>GPLGSKKLKCTVEGCDR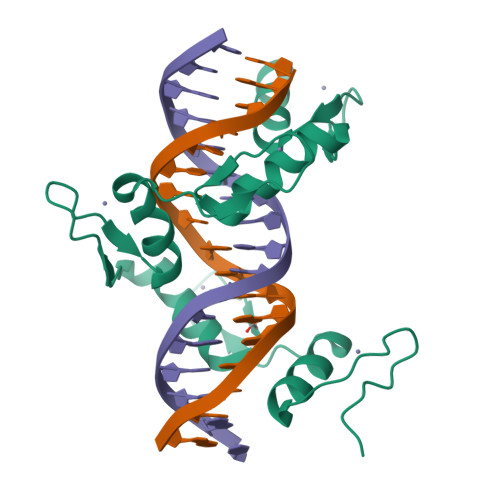TFVWPAHFKYHLKTHRNDRSFICPAEGCGKSFYVLQRLKVHMRTHNGEKPFMCHESGCGKQFTTAGNLKNHRRIHTGEKPFLCEAQGCGRSFAEYSSLRKHLVVHSGEKPHQCQVCGKTFSQSGSRNVHMRKHHLQLG[2x]> MIRAVFFDSLGTLISVEGAYKVRLKIMEEVLGDYPLNPATLLDEYEKLAREAFSNYAGKPYRPMRDILEEVMRKLAEKYGFKYPENLREISLRMACRYGELYPEVVEVLKSLKGKYHVGDILQRDTEPATAFLDALGIKDLFDSITTSEEAGFFKPHPRIFELALKKAGVKGEKAVYVGDNPVKDAGGSKNLGMTSILLDRKGEKREFWDKADFIVSDLREVIKIVDELNGQGSLEHHHHHH

SNAr1.3 can operate at a rate of 0.15 s−1, perform more than 4,000 turnovers and can accept a broad range of electrophilic and nucleophilic coupling partners, including those that allow construction of challenging 1,1-diaryl quaternary stereocentres. Biochemical, structural and computational studies provide insights into the catalytic mechanism of SNAr1.3, including the emergence of a halide binding pocket shaped by key catalytic residues Arg124 and Asp125. In summary, we have established a biocatalytic solution to SNAr chemistry, one of the most important classes of transformations in the chemical industry.

We facilitated structural analysis by a K39A mutation at the protein surface, which has negligible impact on activity and improves data resolution. Notably, despite performing evolution with aryl chloride 2, enzyme activity is improved by 3.8-fold and 8.6-fold using the bromide-containing and iodide-containing analogues of 2, respectively (3.67 ± 0.04 and 8.34 ± 0.11 mM−1 min−1). To explore the potential importance of the halide binding site, SNAr1.3 crystals were soaked with substrate 5. The corresponding structure revealed two distinct anomalous signals in close proximity, associated with the iodide substituent, suggesting that the substrate binds with considerable conformational heterogeneity. Notably, the major 5 pose places the halide substituent directly adjacent to the aforementioned halide binding cavity.> GGCGCUGUGUCGCAAUCUGCGAAGGGCGUCGUCGCCCCAAGCGGUAGUAAGCAGGGAACUCACCUCCA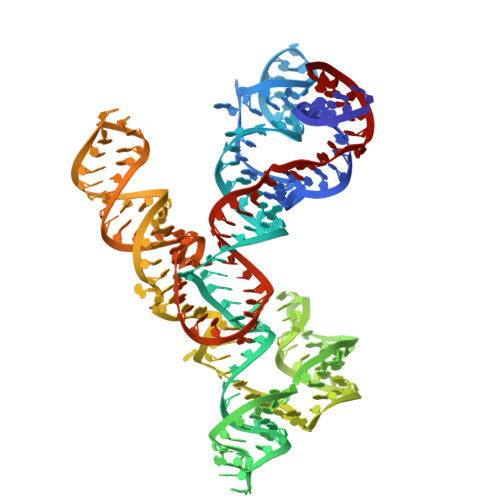AUGAAACACAUUGUCGUAGCAGUUGACUACUGUUAUGUGAUUGGUAGAGGCUAAGUGACGGUAUUGGCGUAAGCCAAUACCGCAGCACAGCACAAGCCCGCUUGCGAGAUUACAGCGC> MTTLLNPYFGEFGGMYVPQILMPALNQLEEAFVRAQKDPEFQAQFADLLKNYAGRPTALTKCQNITAGTRTTLYLKREDLLHGGAHKTNQVLGQALLAKRMGKSEIIAETGAGQHGVASALASALLGLKCRIYMGAKDVERQSPNVFRMRLMGAEVIPVHSGSATLKDACNEALRDWSGSYETAHYMLGTAAG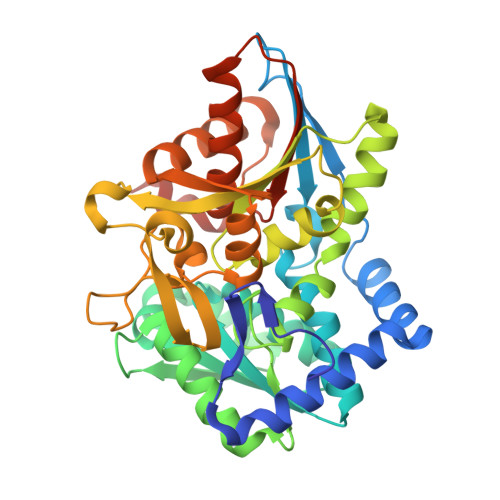PHPYPTIVREFQRMIGEETKAQILDKEGRLPDAVIACVGGGSNAIGMFADFINDTSVGLIGVEPGGHGIETGEHGAPLKHGRVGIYFGMKAPMMQTADGQIEESYSISAGLDFPSVGPQHAYLNSIGRADYVSITDDEALEAFKTLCRHEGIIPALESSHALAHALKMMREQPEKEQLLVVNLSGRGDKDIFTVHDILKARGEI SDRs each have a Rossmann fold for NAD(P)+ binding, and the SDR active site is characterized by a conserved catalytic tyrosine residue, which is accompanied by a lysine residue to give the conserved motif YxxxK; frequently a serine or threonine unit serves as an additional active‐site residue to make a catalytic triad. To investigate whether C. roseus harbours an SDR that uses strictosidine aglycone as a substrate, SDR gene candidates that were co‐regulated with known MIA biosynthetic genes were selected for screening in in vitro biochemical assays. The discovery of VAS demonstrates the capacity of an SDR to reduce an additional isomer of strictosidine aglycone to form a new alkaloid backbone. The reduction catalysed by VAS probably works by a standard SDR mechanism, with the C‐4 hydride of NADPH attacking C‐17 of the iminium substrate.

Crystallization of VAS was carried out with and without the oxidized cofactor NADP+. After solution of the structures it was clear that the apo enzyme active site also had a high occupancy of NADP+, thus indicating that VAS is purified from E. coli as a holoenzyme. The two subunits of VAS in the asymmetric unit form a dimeric assembly. Part of the interface involves an extended loop from each subunit (residues 103–124), delineated by β5 and β6 that form a β‐hairpin, although sections of this loop are disordered in both subunits; this is referred to as the “flap domain” in related structures. The core of each subunit is the canonical Rossmann nucleotide binding fold characteristic of the SDR enzymes, in which the cofactor lies across the end of the central, predominantly parallel, β‐sheet. The two active‐site cavities face each other across the apparent dimer interface, with the two opposing NADP+ C‐4 atoms only ≈17 Å apart, and are framed by the base of the flap domain and another loop that arises between β8 and α9 (residues 251–266) and folds over the cofactor (i.e., the “cofactor loop”). In this arrangement, the active centres are effectively inaccessible to bulk solvent, thus prompting us to speculate that the quaternary structure suggested by the crystal structure is not representative of the active state of the enzyme. In support of this proposal, the elution profiles of VAS in size exclusion chromatography and dynamic light scattering analysis are consistent with a monomeric species with an estimated molecular size of 32 kDa (calculated molecular mass of His6‐VAS is 34 469 Da). The substrate‐binding pocket itself is comparatively constricted, with the C‐4 atom of the nicotinamide ring projecting into it.

>MAHHHHHHSSGLEVLFQGPAAMGTSEKYAVVTGSNKGIGFETCKKLASQGITVVLTARDEKRGLDALEKLKELGLSGKVLFHQLDVTDSSSVASLAEFVKKQFGRLDILVNNAGVNGVITDVEAVKKLNPAEDPADVDFSKIYKETYELAEECIQINYFGTKRTTDALLPLLQLSASPRIVNISSIMGQLKNIPSEWAKGILGDASNLTEDRLDEVINNFLKDFKEGSLAAKGWPPSFSAYIVSKVVVNAYTRILAKKYPNFKINCVCPGFAKTDLNHGLGLLTAEEAAENPVKLALLPDDGPSGLFFDRSEESSFE[2x]>[2x]MGKYNLILSEYLSFIYNSQSAVQIPIYYSSNSELENRCIEFHSKCLENSKNGLSLRKLFVEYNDVIENATLLSILSYSYDKYNAVERKLVKYAKGKPLEADLTVNELDYENNKMTSELFPTAEEYTDSLMDPAILTSLSSNL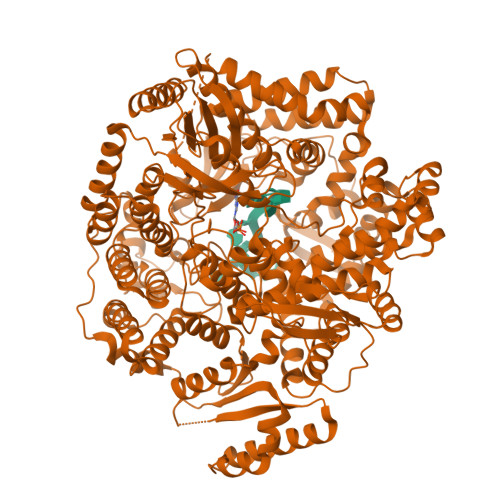NAVMFWLEKHENDVAEKLKVYKRRLDLFTIVASTINKYGVPRHNAKYRYEYDVMKDKPYYLVTWANSSIEMLMSVFSHDDYLIAKELIVLSYSNRSTLAKLVSSPMSILVALVDINGTFITNEELELEFSNKYVRAIVPDQTFDELNQMLDNMRKAGLVDIPKMIQDWLVDRSIEKFPLMAKIYSWSFHVGFRKQKMLDAALDQLKTEYTENVDDEMYREYTMLIRDEVVKMLEEPVKHDDHLLRDSELAGLLSMSSASNGESRQLKFGRKTIFSTKKNMHVMDDMANERYTPGIIPPVNVDKPIPLGRRDVPGRRTRIIFILPYEYFIAQHAVVEKMLIYAKHTREYAEFYSQSNQLLSYGDVTRFLSNNTMVLYTDVSQWDSSQHNTQPFRKGIIMGLDILANMTNDAKVLQTLNLYKQTQINLMDSYVQIPDGNVIKKIQYGAVASGEKQTKAANSIANLALIKTVLSRISNKHSFATKIIRVDGDDNYAVLQFNTEVTKQMIQDVSNDVRETYARMNAKVKALVSTVGIEIAKRYIAGGKIFFRAGINLLNNEKRGQSTQWDQAAILYSNYIVNRLRGFETDREFILTKIMQMTSVAITGSLRLFPSERVLTTNSTFKVFDSEDFIIEYGTTVDEVYIQRAFMSLSSQKSGIADEIAASSTFKNYVTRLSEQLLFSKNNIVSRGIALTEKAKLNSYAPISLEKRRAQISALLTMLQKPVTFKSSKITINDILRDIKPFFTVSDAHLPIQYQKFMPTLPDNVQYIIQCIGSRTYQIEDDGSKSAISRLISKYSVYKPSIEELYKVISLHENEIQLYLISLGIPKIDADTYVGSKIYSRDKYRILESYVYNLLSINYGCYQLFDFNSPDLEKLIRIPFKGKIPAVTFILHLYAKLEVINYAIKNGSWISLFCNYPKSEMIKLWKKMWNITSLRSPYTNANFFQEPHHHHHH(6R)-6-[(1R,3aS,4E,7aR)-7a-methyl-4-[2-[(3R,5R)-4-methylidene-3,5-bis(oxidanyl)cyclohexylidene]ethylidene]-2,3,3a,5,6,7-hexahydro-1H-inden-1-yl]hept-1-en-3-one 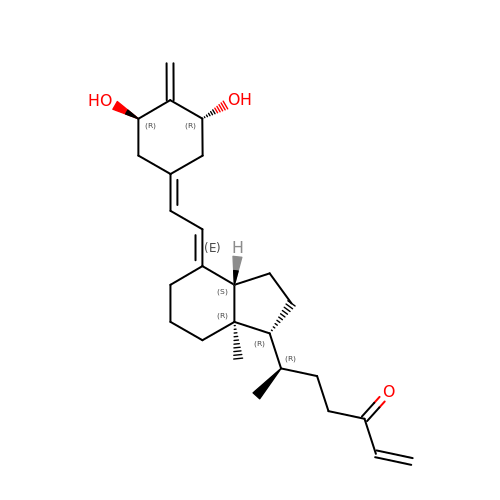| C26 H38 O3 | XVGVVMUDYCUDFM-VMKNJNNYSA-N>[6x]MHHHHHHMLENKLGIINQLELNRVEERVSKENAKRLYDSGDIDRIEVGTFKGLSYIHNYLFEDIYEFAGKVRSQNI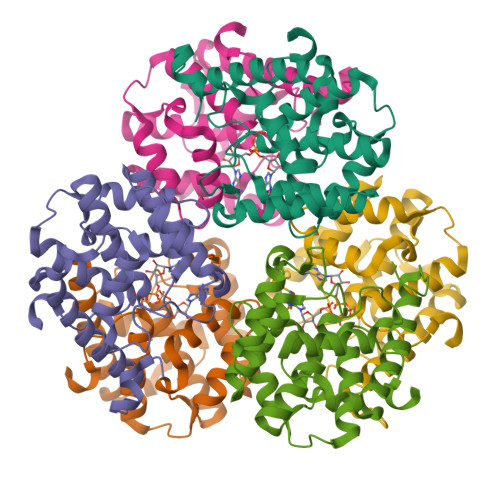SKGNFRFAPVMYLEIALEHIDKMPQRNLDEIVAKYVEMNIAHPFREGNGRATRIWLDLILKKELKRVVDWNLINKEDYLSAMERSPVKDLEIKYLISNALTDKINDREIFMKGIDISYYYEGYTEYNVDEL>[4x]MADLNWISSALIKERPSADAVLAKAVLAAREQLGLTQLELAGIVGVDRSAISRWKTQGLRVDSKTGELALLLVRVYRALYALFGGQQEDMRHFLRTPNHHLAGEPLALMGQVQGLVHVLEYLDAIRGKV;>[2x]MGSSHHHHHHSQDPSEIWRQCKGERHIRPLQGRLVRLVESQDQVATLQLVDTLEEQALLEELLESSKPPVPADAEPLHYLLKTPFRYPPLRWGSRFGRRHEPSLFYAALKLETAMAESAYYRCVLWSGMVVPPPSGRILSEHASFEAGWKVERGIRLQAPPFSDHEAALTDIADYRAPQELGSAMRSAGVQAFEYRSARCPERGCNVALFTPAAFTEKRPRNLTPWLCETTAGYVAFKPAHVPGSPKIFSWELFLVDGKLPHPA

Here, we show that the NatR–NatT TA system, which is part of the core genome of the human pathogen Pseudomonas aeruginosa, generates drug-tolerant persisters by specifically depleting nicotinamide dinucleotides. We show that NatT is an NAD phosphorylase, which leads to the depletion of both NAD and NADP in a subpopulation of cells. NatT function is tightly controlled by NatR, which is both an anti-toxin and an auxiliary factor required for toxin stability. NatT belongs to a subgroup of RES domain proteins that have adopted a Flap region mediating its interaction with the anti-toxin NatR.

Ectopic expression of natTE29D, a mutant isolated in a screen for increased tolerance in P. aeruginosa, showed stronger interference with growth (Fig. EV1D) and strongly increased survival during exposure to tobramycin (Fig. EV1E) or ciprofloxacin (Fig. EV1F). Thus, the E29D mutation boosts toxin-associated phenotypes, suggesting that it unleashes NatT activity. To explore the NatT activation mechanism, we next solved the structure of NatTE29D in complex with NatR. Structural differences between wild-type and mutant proteins were limited to subtle changes in the NatR’-NatT interface close to residue E29. A water molecule bridging the phosphate positioned in the NatR’-NatT interface with residues T70 and R73 of NatT wild-type was missing in the E29D mutant. Moreover, the E29D substitution changes its interaction with R119 of NatR’, forcing the neighboring E26 to adopt a different rotameric configuration, which in turn disrupts the interaction with the main chain of the C-terminal helix α7 of NatR’. Based on this, we speculate that the E29D mutation weakens the interaction between the NatT Flap and NatR’, thereby promoting the disassembly of the stable hexameric structure. Thus, the activating mutation E29D may not only disturb the interaction between the Flap and helix α7, but may also disrupt NatT dimerization. Importantly, the NatR–NatTE29D complex showed a single peak at 60 kDa, indicating that the TA complex is in a dynamic equilibrium between an inert hexameric state and a smaller, active subcomplex and that this transition mediates NatT toxin activation. In agreement with this, purified NatR–NatT wild-type complex (4R:2T) readily bound to the natR–natT promoter region, while a purified NatTE29D complex failed to bind the same DNA fragment.> MGSDKIHHHHHHENLYFQGMDVGMPFSGPVSFPLLVIEEELPFRIHNICSETGKFDVVLDSITNMPKYGLKIFAGVRIDMYSILGDESSGRIYTLRKGTLADFNARILAYYDKAQVINADGDTCIKMANEGYSALVGNEISIGKSFRNRMKELGLDLPSCAMASTR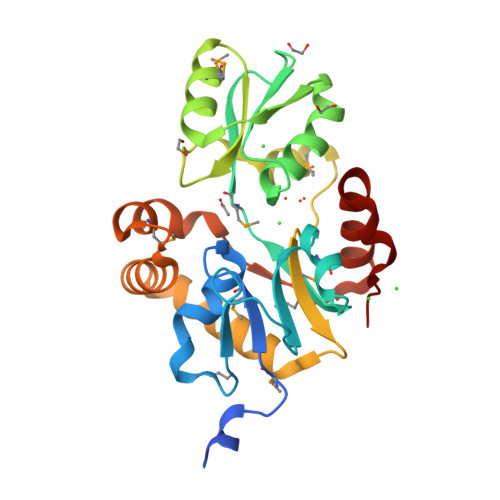RIDEVIEAYEQGIDFIKNNHERAAEIISKKSGYYSEEVMKKIIGIYGHEVTKKRAELVGSRELYSRVVPELNDIEIIG>RKTGLKQKIVIKVAMEGNNCRSKAMALVASTGGVDSVALVGDLRDKIE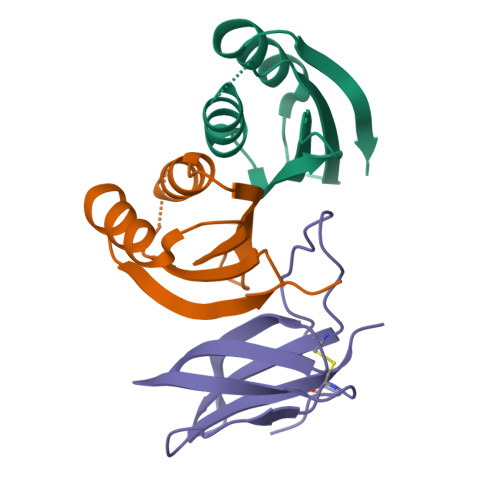VVGYGIDPIKLISALRKKVGDAELLQVSQAKED[4x];>[2x]METGNKYIEKRAIDLSRERDPNFFDNPGIPVPECFWFMFKNNVRQDDGTCYSSWKMDMKVGPNWVHIKSDDNCNLSGDFPPGWIVLGKKRPGF>[4x]MHHHHHHLPNITILATGGDIAGGGDSATKSNYTVGKVGVENLVNAVPQLKDIANVKGEQVVNIGSQDMNDNVWLTLAKKINTDCDKTDGFVITHGTDTMEETAYFLDLTVKCDKPVVMVGAMRPSTSMSADGPFNLYNAVVTAADKASANRGVLVVMNDTVLDGRDVTMTNTTDVATFKSVNYGPLGYIHN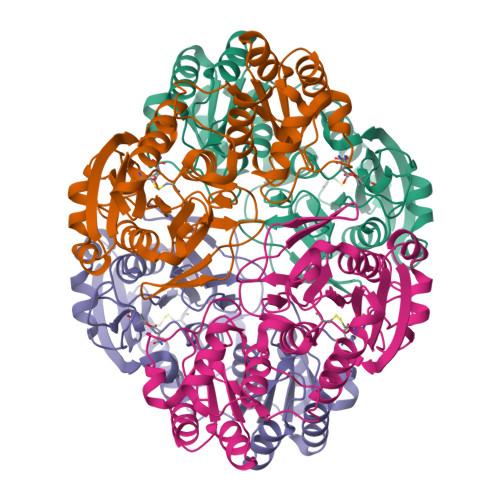GKIDYQRTPARKHTSDTPFDVSKLNELPKVGIVYNYANASDLPAKALVDAGYDGIVSAGVGNGNLYKSVFDTLATAAKTGTAVVRSSRVPTGATTQDAEVDDAKYGFVASGTLNPQKARVLLQLALTQTKDPQQIQQIFNQY(3~{R},4~{R})-1,1-bis(oxidanylidene)thiolane-3,4-diol | C4 H8 O4 S | 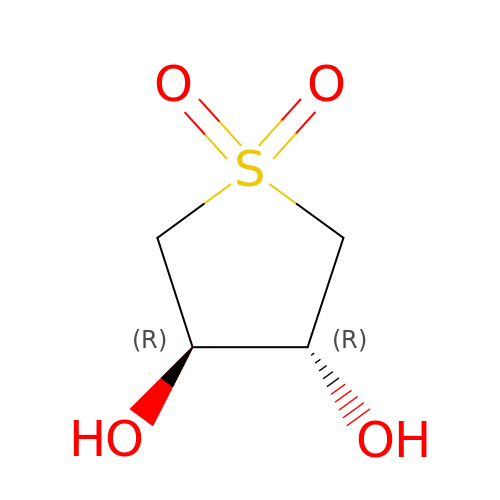LDVDYVUZEKIBDP-IMJSIDKUSA-N> MGPSLDFALSLLRRNIRQVQTDQGHF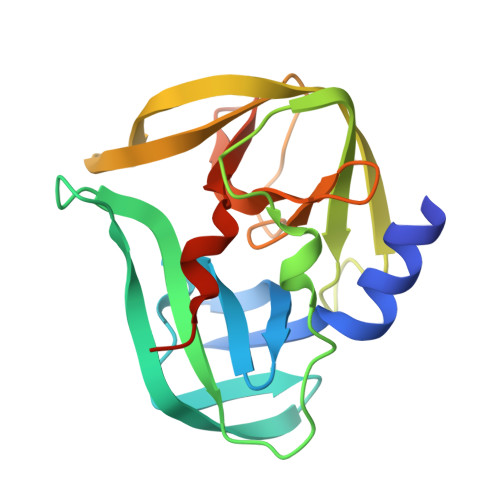TMLGVRDRLAILPRHSQPGKTIWVEHKLINVLDAVELVDEQGVNLELTLVTLDTNEKFRDVTKFIPETITGASDATLIINTEHMPSMFVPVGDVVQYGFLNLSGKPTHRTMMYNFPTKAGQCGGVVTSVGKIIGIHIGGNGRQGFCAGLKRGYFASEQHHHHHH> AKCVSYGVSQIKAPALHSQGYTGSNVKVAVIDSGIDSSHPDLNVAGGASFVPSETNPFQDNNSHGTHVAGTVLAVAPSASLYAVKVLGADGSGQYSWIINGIEWAIANNMDVINMSLGGPSGSAALKAAVDKAVASGVVVVAAAGNEGTSGSSSTVGYPGKYPSVIAVGAVDSSNQRASFSSVGPELDVMAPGVSICSTLPGNKYGAKSGTSMASPHVAGAAALILSKHPNWTNTQVRSSLENTTTKLGDSFYYGKGLI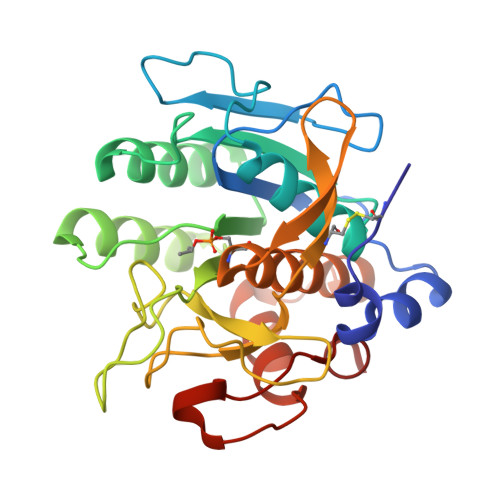NVEAAAQ> GPVEESVERAMVRVADTVSSKPTNSESIPALTAAETGHTSQVVPSDTMQTRHVKNYHSRSESSIENFLCRSACVYYATYNNNSEKGYAEWVINTRQVA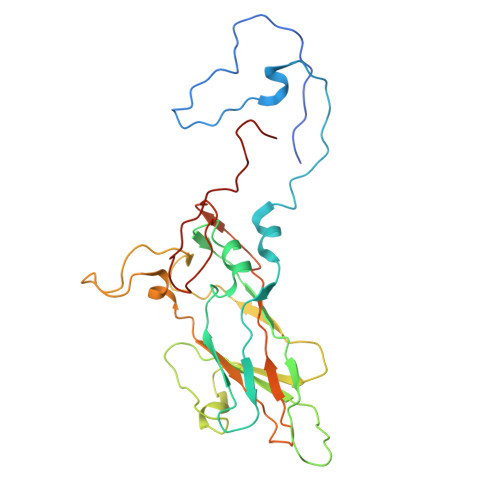QLLRRKLEFTYLRFDLELTFVITSAQEPSTATSVDAPVQTQQIMYVPPGGPVPTKVTDYAWQTSTNPSVFWTEGNAPPRMSIPFISIGNAYSCFYDGWTQFSRNGVYGINTLNNMGTLYMRHVNEAGQGPIKSTVRIYFKPKHVKAWVPRPPRLCQYEKQKNVNFNPTGVTTTRSNITTT>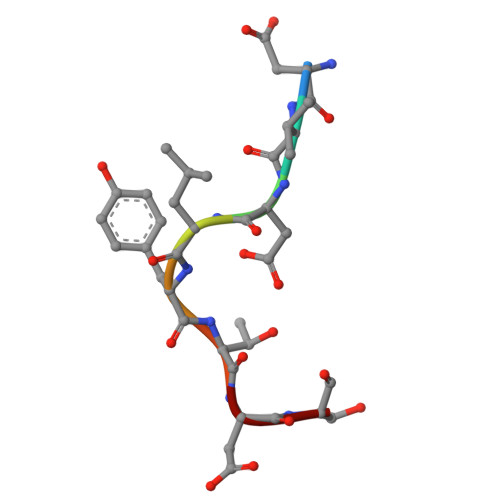 DVDLYTDS> MHHHHHHMMLEAKFEEASLFKRIIDGFKDCVQLVNFQCKEDGIIAQAVDDSRVLLVSLEIGVEAFQEYRCDHPVTLGMDLTSLSKILRCGNNTDTLTLIADNTPDSIILLFEDTKKDRIAEYSLKLMDIDADFLKIEELQYDSTLSLPSSEFSKIVRDLSQLSDSINIMIT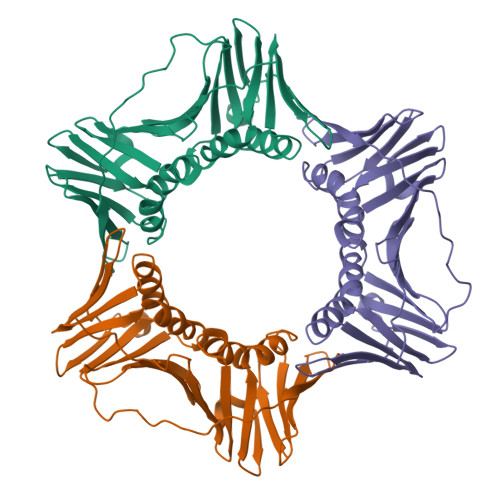KETIKFVADGDIGSGSVIIKPFVDMEHPETSIKLEMDQPVDLTFGAKYLLDIIKGSSLSDRVGIRLSSEAPALFQFDLKSGFLQFFLAPKFNDEE> FNCTSSSATVHWLGDKPTYHAGVTFGLPWPQGKYRPQETSFSLTGDTEDKSELQSWATGYWADGSLKWTAHAIAESNQIYDQYTVTASSLGCVKSSSSSSESSAPNSSIVVTDNSDALTVNTGEVAVSFPKGGNVIIGDIKTKSGKVIGANGRLVLQSQDSVPDNFDNRANSPIQYSNFDGNINEVFVNQTSARTLVTVRGNHTVTDGTDHDPWLPFVVRFYLYANSATIKVMHSIVFDGDENDFITGLGIRFDVPLKGEEYYDRHIRFAGVDGGIFNEAVQGITGLRRDPGEEIRAAQFAGQKLADTETWEPRVSTRLKWIPTWADYGLTQLTADGFGLKKRTKAGQSWVNIPSGTRAEGLAYLGGATQGGLAVGLRDFWKRYPVGLDISNAASDTGELTLWLYSPAAEPLDLRPFHDGLGQDGYEDQLDALEITYEDWEPGFDTPYGIARTSEVYLFAFDQTPTSDKLASLTAYMNDPPVLVAEPKYIHETQALGEYWALPGSASPAAATLEDRLQFIFDFYKGQIEQRRWYGFLDYGDFMHTYDPDRHTWRYDVGGYAWDNSELSPDLFFWLYFLRTGSKDAYRFAEALTRHTGEVDVYHIGDWKGLGTRHGVQHWSDSAKQARISQPQYRKYFFYLSGGDERVGELLEELLDTDKTYGELDPQRKVRTDGWEPSPNSTVSFGLGTDWSGLAAGWLIEWERRGPRWEEAKTKLTNTIAGIANLTNGFVTGSGLYDPVTWTLGPPPSDPGNRGNVSISHLNAVFGLPEVVSEAIAYLADDIPKGFKQAWLDYCYYYHASASEQKDRYGVSFSKISLLQAHSRLAAYAAYETKNKTLALRAWKDFYASDGLLPDAPWNITHVDGSDVLVPVDEAAWLATNDIAQYGLAVIQNLAYVSDSLDDYQSLE;> FNCTSSSATVHWLGDKPTYHAGVTFGLPWPQGKYRPQETSFSLTGDTEDKSELQSWATGYWADGSLKWTAHAIAESNQIYDQYTVTASSLGCVK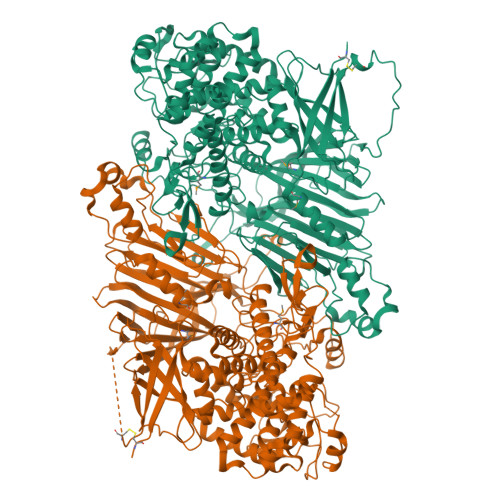SSSSSSESSAPNSSIVVTDNSDALTVNTGEVAVSFPKGGNVIIGDIKTKSGKVIGANGRLVLQSQDSVPDNFDNRANSPIQYSNFDGNINEVFVNQTSARTLVTVRGNHTVTDGTDHDPWLPFVVRFYLYANSATIKVMHSIVFDGDENDFITGLGIRFDVPLKGEEYYDRHIRFAGVDGGIFNEAVQGITGLRRDPGEEIRAAQFAGQKLADTETWEPRVSTRLKWIPTWADYGLTQLTADGFGLKKRTKAGQSWVNIPSGTRAEGLAYLGGATQGGLAVGLRDFWKRYPVGLDISNAASDTGELTLWLYSPAAEPLDLRPFHDGLGQDGYEDQLDALEITYEDWEPGFDTPYGIARTSEVYLFAFDQTPTSDKLASLTAYMNDPPVLVAEPKYIHETQALGEYWALPGSASPAAATLEDRLQFIFDFYKGQIEQRRWYGFLDYGDFMHTYDPDRHTWRYDVGGYAWDNSELSPDLFFWLYFLRTGSKDAYRFAEALTRHTGEVDVYHIGDWKGLGTRHGVQHWSDSAKQARISQPQYRKYFFYLSGGDERVGELLEELLDTDKTYGELDPQRKVRTDGWEPSPNSTVSFGLGTDWSGLAAGWLIEWERRGPRWEEAKTKLTNTIAGIANLTNGFVTGSGLYDPVTWTLGPPPSDPGNRGNVSISHLNAVFGLPEVVSEAIAYLADDIPKGFKQAWLDYCYYYHASASEQKDRYGVSFSKISLLQAHSRLAAYAAYETKNKTLALRAWKDFYASDGLLPDAPWNITHVDGSDVLVPVDEAAWLATNDIAQYGLAVIQNLAYVSDSLDDYQS Among them, Oligoribonuclease (Orn) is unique as its activity is required for clearing short RNA fragments, which is important for cellular fitness. Here, we show that Orn exhibits exquisite substrate preference for diribonucleotides. While other cellular RNases process oligoribonucleotides down to diribonucleotide entities, Orn is the one and only diribonucleotidase that completes the terminal step of RNA degradation. From this we propose a general model of RNA degradation, wherein a combination of exoribonucleases process oligoribonucleotides down to diribonucleotides and Orn completes RNA recycling by cleaving diribonucleotides to nucleoside monophosphates.

We initially determined the crystal structure of P. aeruginosa Orn (OrnPa) with diribonucleotide substrate; however, crystal packing contacts prevented substrate binding (data not shown). Instead, we were able to crystallize two representative homologs, OrnVc and the human REXO2 (also known as small fragment nuclease or Sfn [Bruni et al., 2013]), bound to the diribonucleotide pGpG (Figure 2—source data 1). Superimposing the two structures indicates their identical fold (rmsd of 0.75 Å for the protomer), which is preserved in the substrate-free Orn structure determined previously (rmsd of 0.54 Å for the protomer). The pGpG-bound structures reveal a narrow active site that is lined by the conserved acidic residues of the signature DEDD motif (D12, E14, and D112 of OrnVc; D15, E17, and D115 of REXO2) and the general base H158 or H162 in OrnVc or REXO2, respectively (Figure 2A and B and Figure 2—figure supplement 1B and Figure 2—source data 2). Residue numbering for REXO2 refers to its cytosolic isoform lacking the mitochondria-targeting pre-sequence. The corresponding residues, W64 and Y132, are conserved in REXO2. Most notably, residues S108, R130, S135 and the hydroxyl group on Y129 (S111, R133, S138, and Y132 in REXO2) form hydrogen bonds with the 5' phosphate of pGpG, capping the substrate. This phosphate cap creates a major constriction of the active site, which is not observed in structurally related 3'−5' exoribonucleases such as RNase T or ExoI (Figure 2C and Figure 2—figure supplement 1 and Figure 2—source data 2). RNase T and ExoI accommodate longer RNA substrates, facilitated by an expansive active site.

>MAAGESMAQRMVWVDLEMTGLDIEKDQIIEMACLITDSDLNILAEGPNLIIKQPDELLDSMSDWCKEHHGKSGLTKAVKESTITLQQAEYEFLSFVRQQTPPGLCPLAGNSVHEDKKFLDKYMPQFMKHLHYRIIDVSTVKELCRRWYPEEYEFAPKKAASHRALDDISESIKELQFYRNNIFKKKIDEKKRKIIENGENEKTVS[2x]(5aS,12aS,13aS)-9-chloro-12,12-dimethyl-2,3,11,12,12a,13-hexahydro-1H,5H,6H-5a,13a-(epiminomethano)indolizino[7,6-b]carbazol-14-one | C21 H24 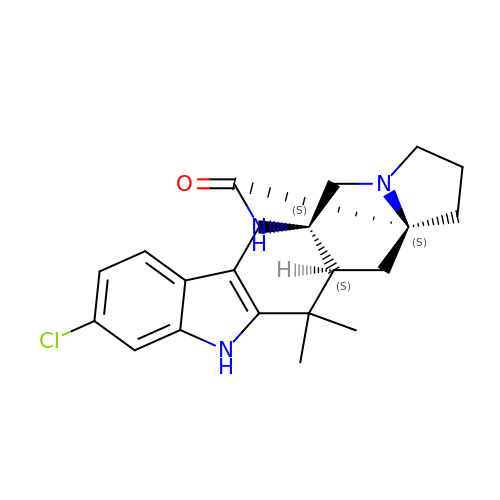Cl N3 O | DXPVAKSJZFQGSS-DQLDELGASA-N>[8x]MAKAVDAAAAAAAAIAPVDTTVVNEDVALVENETCNDQNVQFDSLPSMKYASFLNSDGSVAIHAGERLGRGIVTDAITTPVVNTSAYFFN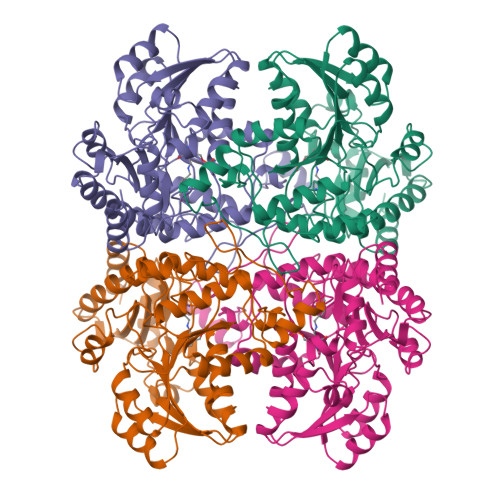KTSELIDFKEKRRASFEYGRYGNPTTVVLEEKISALEGAESTLLMASGMCASTVMLLALVPAGGHIVTTTDCYRKTRIFIETILPKMGITATVIDPADVGALELALNQKKVNLFFTESPTNPFLRCVDIELVSKLCHEKGALVCIDGTFATPLNQKALALGADLVLHSATKFLGGHNDVLAGCISGPLKLVSEIRNLHHILGGALNPNAAYLIIRGMKTLHLRVQQQNSTALRMAEILEAHPKVRHVYYPGLQSHPEHHIAKKQMTGFGGAVSFEVDGDLLTTAKFVDALKIPYIAPSFGGCESIVDQPAIMSYWDLSQSDRAKYGIMDNLVRFSFGVEDFDDLKADILQALDSI> IVGGYTCQENSVPYQVSLNSGYHFCGGSLINDQWVVSAAHCYKSRIQVRLGEHNINVLEGNEQFVNAAKIIKHPNFDRKTLNNDIMLIKLSSPVKLNARVATVALPSSCAPAGTQCLISGWGNTLSSGVNEPDLLQCLDAPLLPQADCEASYPGKITDNMVCVGFLEGGKDSCQGDCGGPVVCNGELQGIVSWGYGCALPDNP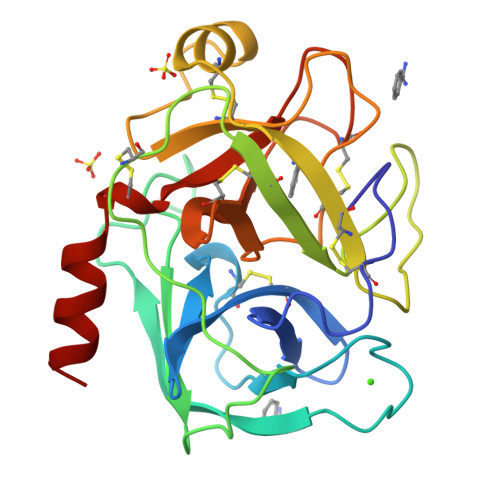GVYTKVCNYVDWIQDTIAAN> MAKRLRVEDDFNPVYPYGYARNQNIPFLTPPFVSSDGFKNFPPGVLSLKLADPITINNGDVSLKVGGGLAVEQQTGNLSVNPDAPLQVASDKLQLALAPPFEVRDGKLALKAGNGLKVLD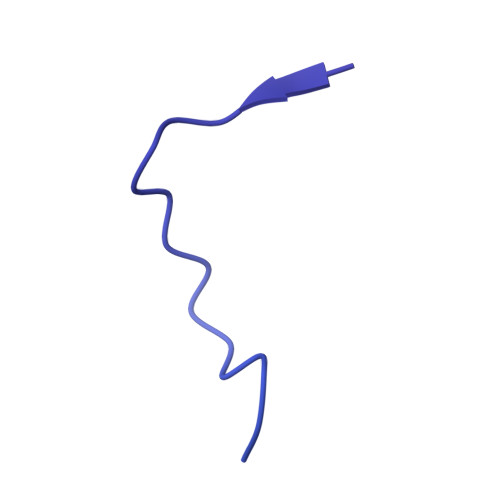NSITGLTGLLNTLVVLTGRGIGTEELKNDDGVTNKGVGLRVRLGDDGGLTFDKKGDLVAWNKKDDRRTLWTTPDTSPNCKMSTEKDSKLTLTLTKCGSQVLGNVSLLAVTGEYHQMTATTKKDVKISLLFDENGILLPSSSLSKDYWNYRSDDSIVSQKYNNAVPFMPNLTAYPKPSAQNAKNYSRTKIISNVYLGALTYQPVIITIAFNQETENGCAYSITFTFTWQKDYSAQQFDVTSFTFSYLTQENKDKD>MTEYEGPKTKFHALMQEQIHNEFTAAQQYVAIAVYFDSEDLPQLAKHFYSQAVEERNHAMMLVQHLLDRDLRVEIPGVDTVRNQFDRPREALALALDQERTVTDQVGRLTAVARDEGDFLGEQFMQWFLQEQIEEVALMATLVRVADRAGANLFELENFVAREVDVAPAASGAPHAAGGRL[24x]

Ferritins are protein complexes that are involved in iron homeostasis and DNA repair by storing iron in cage-like structures. This protein complex is formed by 12 or 24 subunits with tetrahedral 23-symmetric or octahedral 432-symmetric arrangements, depending on the subfamily to which it belongs. Here, a straightforward expression and purification protocol is presented that provides an apoferritin, bacterioferritin B (BfrB), from Mycobacterium tuberculosis with high yield and purity. Similar to as in S. coelicolor bacterioferritin, Fe2+ enters BfrB from the B-pore and is converted to Fe3+ at the ferroxidase centres.

A 2.12 Å resolution cryo-EM structure of BfrB is reported, showing the typical cage-like oligomer constituting of 24 monomers related by 432 symmetry. However, it also contains a unique C-terminal extension (164–181), which loops into the cage region of the shell and provides extra stability to the protein. Part of this region was ambiguous in previous crystal structures but could be built within the cryo-EM map. The C-terminal region 164–181 consists of a flexible part (Cflex, 164–173) and a rigid part (Crigid, 174–181), as described by Khare et al.. We found the extension of the C-terminal end to be located within the interior of the BfrB cage, which is remarkable as Mt-enc has been reported to encapsulate BfrB via this C-terminal extension. Our EM map displays well defined density for Crigid, residues 174–181, including a double conformation of residue His175. We placed water molecules here, as we lack experimental evidence for these water molecules being ions. Both the A and the B site have clear densities, where the A site is coordinated by Glu22 (2.55 Å), Glu55 (2.78 and 2.82 Å), His58 (2.51 Å) and neighbouring water molecules (2.44 and 2.65 Å).> MVFHYTNFVQETNAWWLRRVRPVYCTVLAYYGWWLYDRYYLFGKNATQDIRKDTTEVWEKRAALNKRNWGYNAHYKPELERSMKKVLYADPNYKFPIEWPERYMAET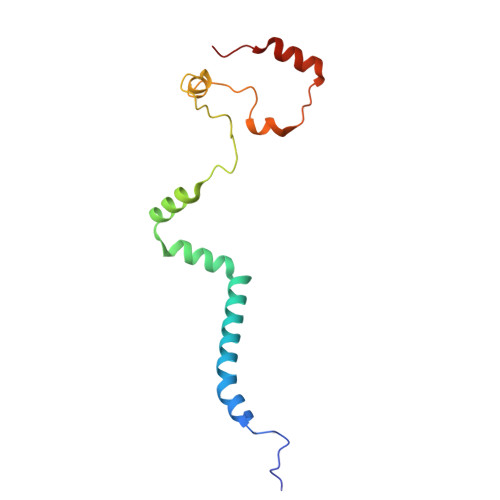KTLEQVMDEEENWEYYK>HHHHHHGSMGYPVIVEATRSPIGKRNGWLSGLHATELLGAVQKAVVDKAGIQSGLHAGDVEQVIGGCVTQFGEQSNNISRVAWLTAGLPEHVGATTVDCQCGSGQQANHLIAGLIAAGAIDVGIACGIEAMSRVGLGANAGPDRSLIRAQSWDIDLPNQFEAAERIAKRRGITREDVDVFGLESQRRAQRAWAEGRFDREISPIQAPVLDEQNQPTGERRLVFRDQGLRETTMAGLGELKPVLEGGIHTAGTSSQIS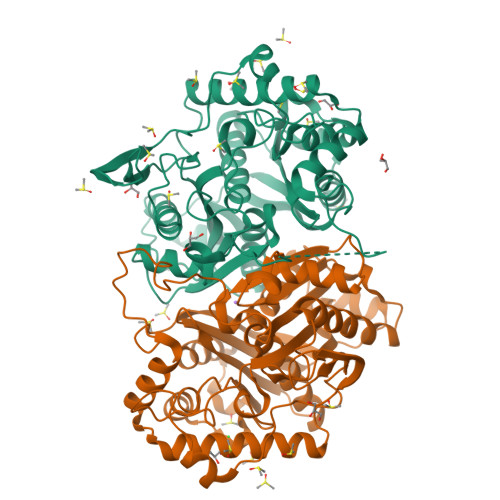DGAAAVLWMDEAVARAHGLTPRARIVAQALVGAEPYYHLDGPVQSTAKVLEKAGMKIGDIDIVEINEAFASVVLSWARVHEPDMDRVNVNGGAIALGHPVGCTGSRLITTALHELERTDQSLALITMCAGGALSTGTIIERI[2x]> AKARDKLEENRDLIVERLKVDEIADFMIEKGELTEEEKKKVDAEDSERKRAEKLVEIVMKMDDAAVKAFYDA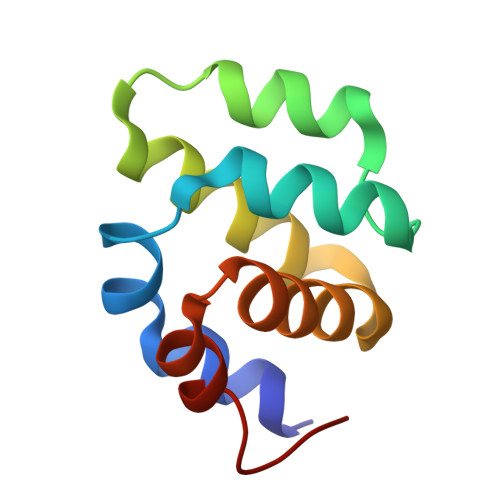LKAKGYSDLASLLESGLC>[2x]ETITVPTPIKQIFSDDAFAETIKDNLKKKSVTDAVTQNELNSIDQIIANNSDIKSVQGIQYLPNVTKLFLNGNKLTDIKPLANLKNLGWLFLDENKVKDLSSLKDLKKLKSLSLEHNGISDINGLVHLPQLESLYLGNNKITDITVLSRLTKLDTLSLEDNQISDIVPLACLTKLQNLYLSKNHISDLRALCGLKNLDVLELFSQEALNKPINHQSNLVVPN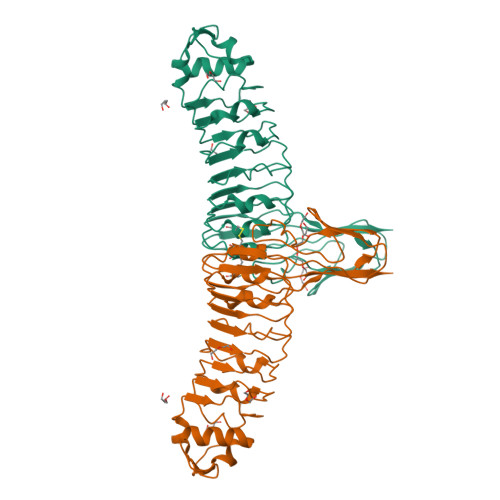TVKNTDGSLVTPEIISDDGDYEKPNVKWHLPEFTNEVSFIFYQPVTIGKAKARFHGRVTQPLKE>[2x]MAPRKFFVGGNWKMNGDKKSLGELIHTLNGAKLSADTEVVCGAPSIYLDFARQKLDAKIGVAAQNCYKVPKGAFTGEISPAMIKDIGAAWVILGHSERRHVFGESDEL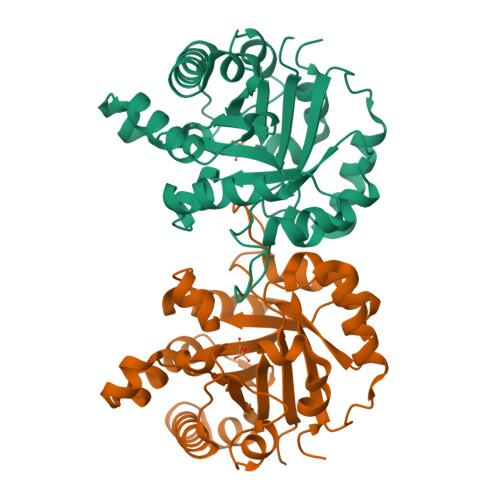IGQKVAHALAEGLGVIACIGEKLDEREAGITEKVVFEQTKAIADNVKDWSKVVLAYEPVWAIGTGLWATPQQAQEVHEKLRGWLKSHVSDAVAQSTRIIYGGSVTGGNCKELASQHDVDGFLVGGASLKPEFVDIINAKH>[4x]SMPPSNFLEIDVSNPQTVGVGRGRFTTYEIRVKTNLPIFKLKESTVRRRYSDFEWLRSELERESKVVVPPLPGKAF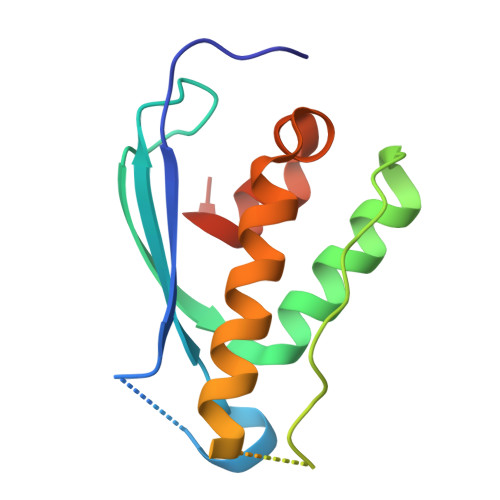LRQLPFRGDDGIFDDNFIEERKQGLEQFINKVAGHPLAQNERCLHMFLQDEIIDKSYT> GLKQKIVIKVAMEGNNCRSKAMALVASTGGVDSVALVGDLRDKIEVVGYGIDPIKLISALRKKVG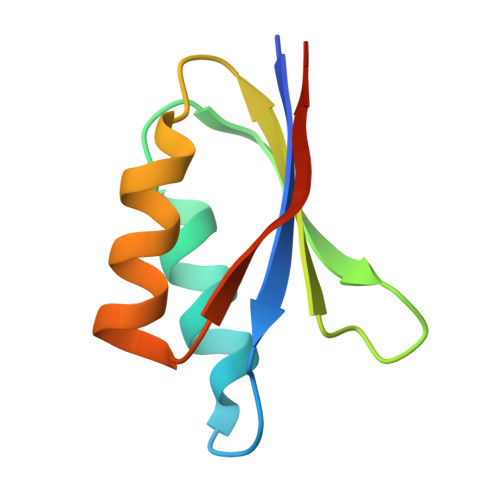DAELLQVSQAKKD N-[5-[[3-(dimethylamino)phenyl]sulfamoyl]-1,3,4-thiadiazol-2-yl]naphthalene-2-carboxamide 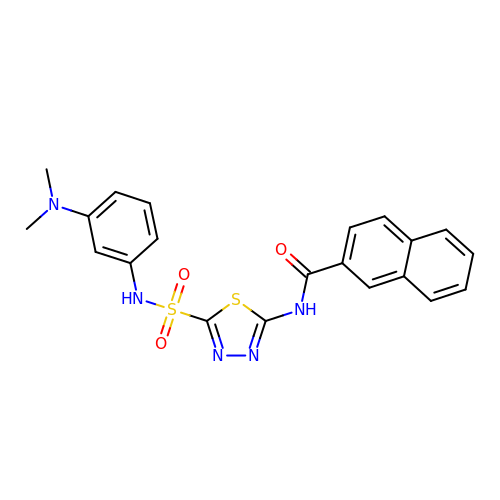| C21 H19 N5 O3 S2 | NBMBYKDETHCBSW-UHFFFAOYSA-N9-DEAZAADENINE 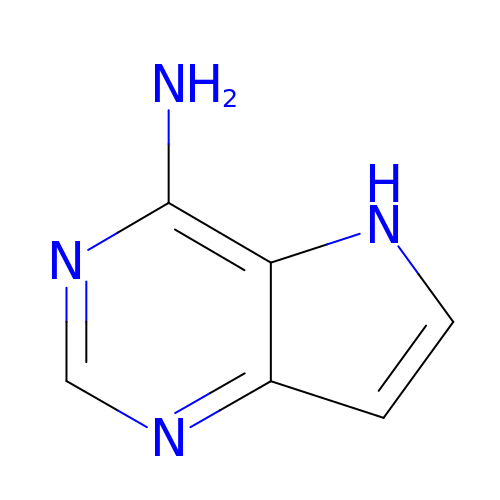| C6 H6 N4 | YRVFQPBPZCRUDX-UHFFFAOYSA-N> 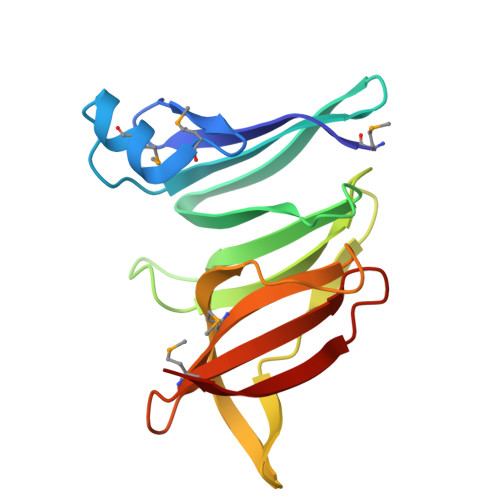MISDFERIREDGKVIDENMTVDQMIALGWSPCRVVEARWRWQEQLLSVVNSRGLLAIVVPDRQHLAILWNDDDTGVAATLYVVSGDRQQQIRIADQLLINGQLEAGIYSWFEQFPQVSPSIFTCMFSRQRDQAMFRVDIDASTGDIVSIQHSR>MKLTENTQPHSPIRLLVVSDNKPLSATLLQCIEALAGDLTVDVDLRYTAYN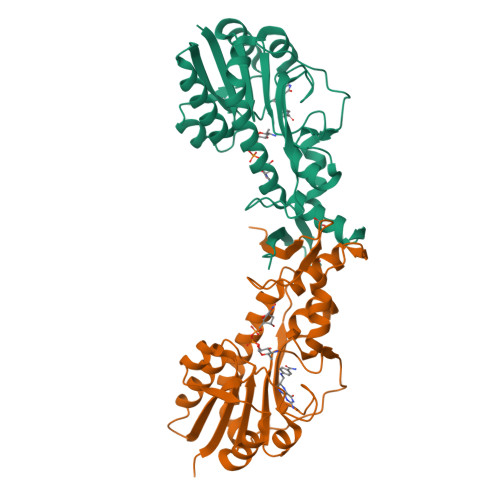HTPQSMVDLGARVIDVKDESVVDLIIEHYDLVLSVHCKQLFPKRLVEGVRCINFHPGFNPFNRGWYPQAFSILNGLPAGATIHVMDEAIDHGHIIVQRQVEVGSGDTSLEVYNKVVEVEKALMHECLADILQGQYEVFKPLSEGNYNGIKAYNELCQLDLEETGSLRDHINLLRATSHGDFKNAYFIDESGDKYFIKVVLEKALRHHHHHH[2x]> HHHHHHSSGLVPRGSHMASMLDMDDLATLDGQNWLNDQVINMYGELIMDAVP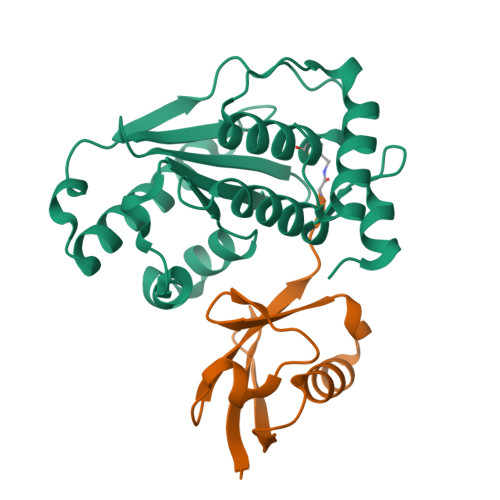DKVHFFNSFFHRQLVTKGYNGVKRWTKKVDLFKKSLLLIPIHLEVHWSLITVTLSNRIISFYDSQGIHFKFCVENIRKYLLTEAREKNRPEFLQGWQTAVTKCIPQQKNDSDCGVFVLQYCKCLALEQPFQFSQEDMPRVRKRIYKELCECRLMD;> MGEYIKLKVIGQDSSEIHFKVKMTTHLKKLKESYCQRQGVPMNSLRFLFEGQRIADNHTPKELGMEEEDVIEVYQEQTGX>[2x]MAVIAFGKFKLNLGTREMFREDEPMPLTSGEFAVLKALVSHPR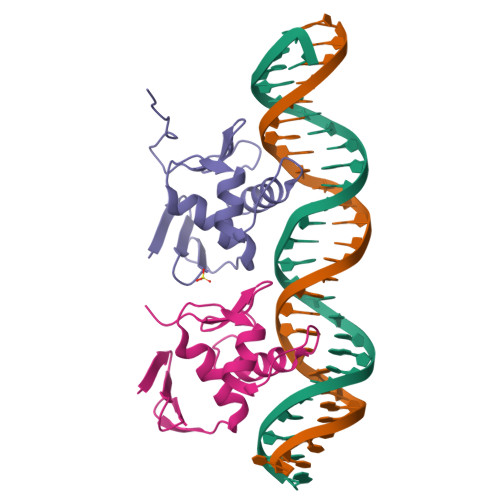EPLSRDKLMNLARGREYSAMERSIDVQISRLRRMVEEDPAHPRYIQTVWGLGYVFVPDGSKALEHHHHHH> PECQITGDR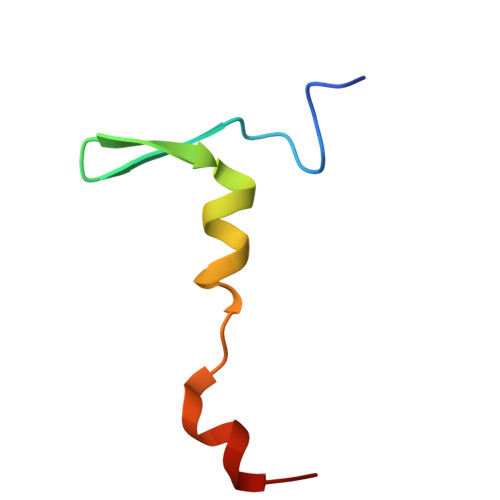PVIKINNTLWESNTAAAFLNRKSQFLYTTGK Here, we report the crystal structures of PhoExo I, which shares 76% amino acid sequence identity with PfuExo I. In this study, we determined three substrate-free structures of PhoExo I and four structures of PhoExo I in complexes with ssDNAs. PhoExo I forms a trimer in solution similar to PfuExo I. The 3′-5′ exonuclease assay of PhoExo I showed that PhoExo I cleaved an ssDNA from its 3′-end at every two nucleotides, and the cleavage stopped at the third to fifth nucleotide from the 5′-end. PhoExo I is predicted to utilize a DEDE (RNase HIII)-type catalytic motif for the hydrolysis of ssDNA. PhoExo I is a novel RNase H superfamily protein.

In this study, we determined three substrate-free PhoExo I structures using three crystals with different unit-cell parameters (crystals 1–3). Crystals 1 and 2 contained one PhoExo I trimer in the asymmetric unit. The protomer structures of the three crystals were nearly identical. Although the protomer structures of each trimer are nearly identical, the trimeric structures are not identical. When the trimeric structures of the three PhoExo I crystals were superposed, the N-terminal half of PhoExo I, especially the α2 and α3 helices, exhibited a structural difference, although the C-terminal half of PhoExo I, which is mainly used for trimerization, was nearly identical between the crystals. In addition, the α2 and α3 helices were partially disordered in the PhoExo I structures in crystals 1 and 2. These data suggest that the trimeric structure of PhoExo I is relatively flexible at its N-terminal half in solution. In the structures of PhoExo I, each PhoExo I protomer binds one Mg2+ ion among the β1 strand of the large β sheet, the α1 helix, the β4–β5 loop and the longest α4 helix. The Mg2+ ion is coordinated by Asp7, Asp80 and four water molecules in an octahedral manner.

>[3x]MRIVAADTGGAVLDESFQPVGLIATVAVLVEKPYKTSKRFLVKYADPYNYDLSGRQAIRDEIELAIELAREVSPDVIHLDSTLGGIEVRKLDESTIDALQISDRGKEIWKELSKDLQPLAKKFWEETGIEIIAIGKSSVPVRIAEIYAGIFSVKWALDNVKEKGGLLVGLPRYMEVEIKKDKIIGKSLDPREGGLYGEVKTEVPQGIKWELYPNPLVRRFMVFEITSKS> MLSPKAATLAERSAGLAFSLYQAMAKDQAVENILLSPVVVASSLGLVSLGGKATTASQAKAVLSAEQLRDEEVHAGLGELLRSLSNSTARNVTWKLGSRLYGPSSVS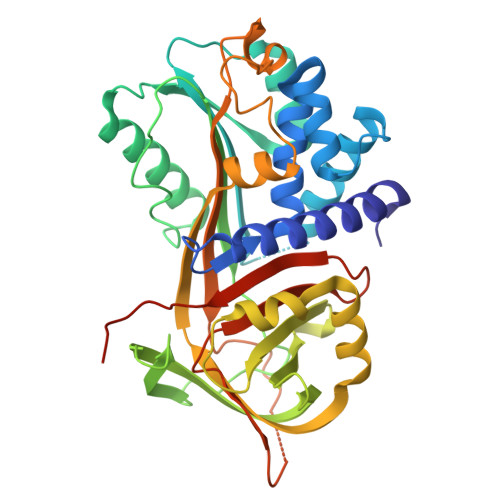FAEDFVRSSKQHYNCEHSKINFRDKRSALQSINEWAAQTTDGKLPEVTKDVERTDGALLVNAMFFKPHWDEKFHHKMVDNRGFMVTRSYTVGVTMMHRTGLYNYYDDEKEKLQIVEMPLAHKLSSLIILMPHHVEPLERLEKLLTKEQLKIWMGKMQKKAVAISLPKGVVEVTHDLQKHLAGLGLTEAIDKNKADLSRMSGKKDLYLASVFHATAFEWDTEGNPFDQDIYGREELRSPKLFYADHPFIFLVRDTQSGSLLFIGRLVRPKGDKMRDELLEHHHHHH>[2x]ELKFLVVDDNSTMRRITRNLLKELGFNNVEEAEDGVD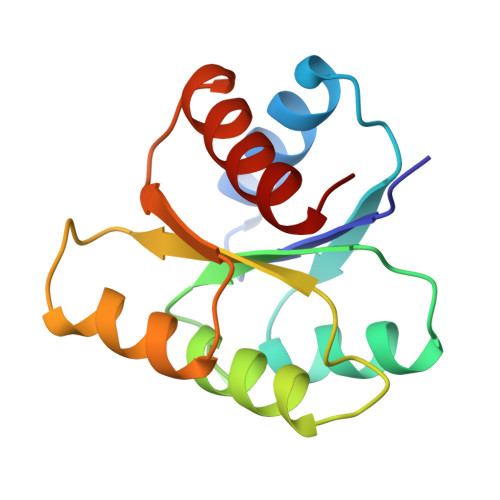ALNKLQAGGYGFVISDWNMPNMDGLELLKTIRADGAMSALPVLMVTAEAKKENIIAAAQAGASGYVVKPFTAATLEEKLNKIFEKLGM>[6x]MPMISCDMRYGRTDEQKRALSAGLLRVISEATGEPRENIFFVIREGSGINFVEHGEHLPDYVPGNANDKALIAKLK;>PFI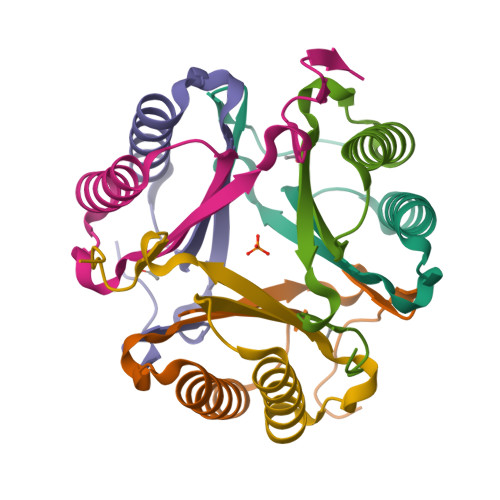ECHIATGLSVARKQQLIRDVIDVTNKSIGSDPKIINVLLVEHAEANMSISGRIHGEAASTERTPAVS[6x]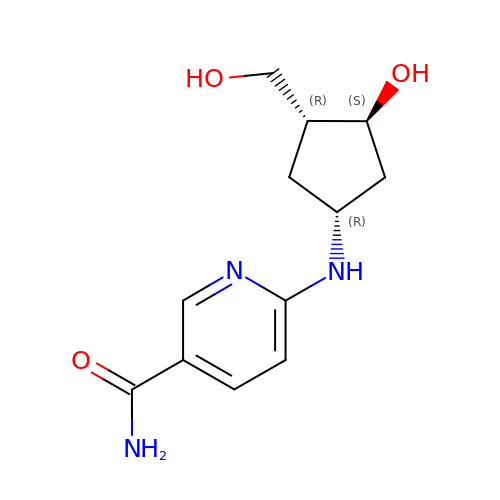6-{[(1R,3S,4R)-3-hydroxy-4-(hydroxymethyl)cyclopentyl]amino}pyridine-3-carboxamide | C12 H17 N3 O3 | OOPBXYPWRQVSFZ-BBBLOLIVSA-N> MIDLSKTVFYTSIDIGSRYIKGLVLGKRDQEWEALAFSSVKSRGLDEGEIKDAIAFKESVNTLLKELEE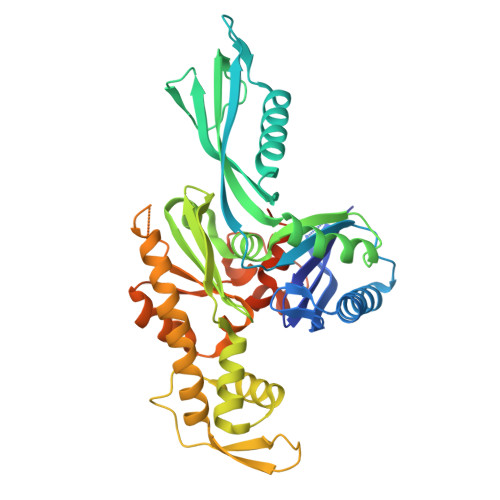QLQKSLRSDFVISFSSVSFEREDTVIERDFGEEKRSITLDILSEMQSEALEKLKENGKTPLHIFSKRYLLDDERIVFNPLDMKASKIAIEYTSIVVPLKVYEMFYNFLQDTVKSPFQLKSSLVSTAEGVLTTPEKDRGVVVVNLGYNFTGLIAYKNGVPIKISYVPVGMKHVIKDVSAVLDTSFEESERLIITHGNAVYNDLKEEEIQYRGLDGNTIKTTTAKKLSVIIHARLREIMSKSKKFFREVEAKIVEEGEIGIPGGVVLTGGGAKIPRINELATEVFKSPVRTGCYANSDRPSIINADEVANDPSFAAAFGNVFAVSENPYEETPVKSENPLKKIFRLFKELME> PTVFHKRYLKKIRDLGEGHFGKVSLYCYDPTNDGTGEMVAVKALKADCGPQHRSGWKQEIDILRTLYHEHIIKYKGCCEDQGEKSLQLVMEYVPLGSLRDYLPRHSIGLAQLLLFAQQICEGMAYLHAQHYIHRDLAARNVLLDNDRLVKIGDFGLAKAVPEGHEYYRVREDGDSPVFWYAPECLKEYKFYYASDVWSFGV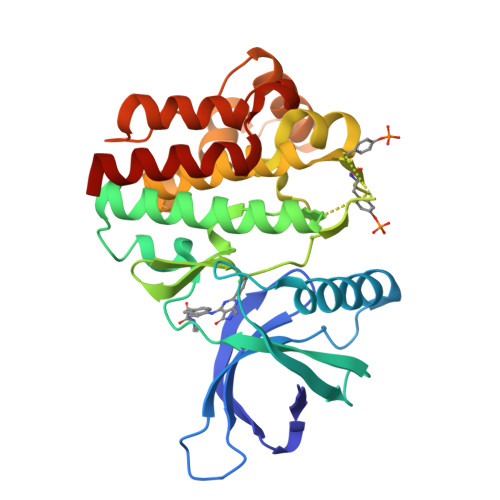TLYELLTHCDSSQSPPTKFLELIGIAQGQMTVLRLTELLERGERLPRPDKCPCEVYHLMKNCWETEASFRPTFENLIPILKTVHEKYQ>GNIRYSVPEETDKGSFVGSIAKDLGLETRELMERGIRIVSRGRSQLFSLNPRSGSLVTAGRIDREELCAQSTPCVVSFNILMEDEMKLLPIEVEIIDINDNTPQFQLEELELKMSEITTPGTRIPLPLGQDLDVGINSLQSYQLSANPHFSLDVQQGPEGPQQPEMVLQRPLDREKDAVHYLVLTASDGGSPIHSGTLQIHVQVVDVNDNPPAFTKAEYHVSVPENVPLGTRLLKVNATDPDEGANGRVTYSFHKVDHSVVRKFQLDAY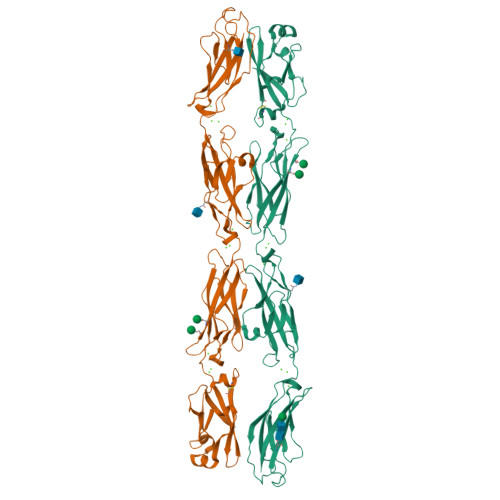TGELSNKEPLDFEEYKVYPMEIQAQDGAGLMARAKVLVTVLDVNDNAPEVGITSVTNTVPENFPPGTTIALISVHDQDADNNGHITCSIPGNLPFKLEKLVDNYYRLVTERTLDREQSSRHNITITATDQGTPPLSTQAHISLLVTDINDHHHHHHHH[4x]(6aR,10aR)-3-(8-bromanyl-2-methyl-octan-2-yl)-6,6,9-trimethyl-6a,7,10,10a-tetrahydrobenzo[c]chromen-1-ol 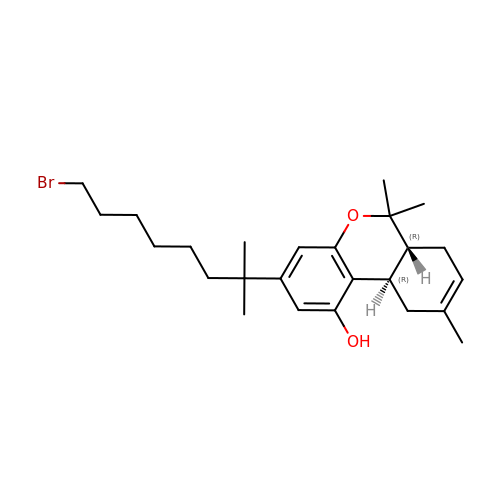| C25 H37 Br O2 | SZDVFUZKFPGYEK-WOJBJXKFSA-N N-(4-((2-((4-(4-methylpiperazin-1-yl)phenyl)amino)-7H-pyrrolo[2,3-d]pyrimidin-4-yl)oxy)phenyl)acrylamide | C26 H27 N7 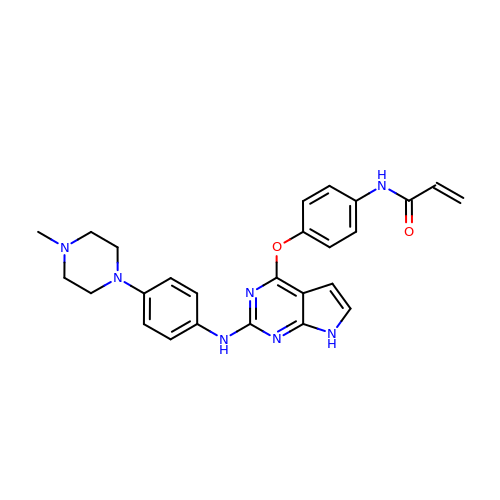O2 | LPJIGUIJJBQRTQ-UHFFFAOYSA-N>GISEFKNSLFVLPYEQRDALNSLISGISSARESVKIAIYSFTHRDIARAIKSVASRGIKVQIIYDYESNHNNKQSTIGYLDKYPNTKV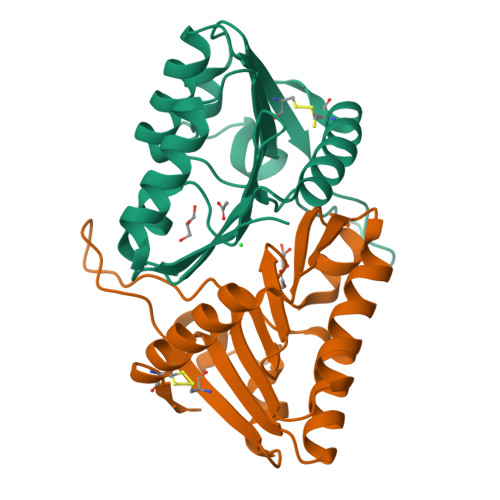CLLKGLKAKNGNYYGIMNQKVAIIDDKIVFLGSANWSKNAFENNYEVLLKTDDTETILKAKSYYQKMLESCVGF[12x]3-[(6-{2-[(3R)-4-(hydroxyacetyl)-3-methylpiperazin-1-yl]pyrimidin-5-yl}-2,2-dimethyl-3-oxo-2,3-dihydro-1H-indol-1-yl)methyl]pyridine-2-carbonitrile 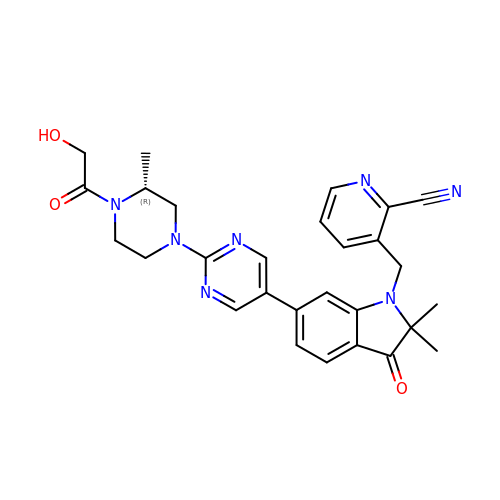| C28 H29 N7 O3 | BTHCNWXORDNTOR-GOSISDBHSA-N>[4x]MPFVNKQFNYKDPVNGVDIAYIKIPNVGVMQPVKAFKIHNKIWVIPERDTFTNPEEGDLNPPPEAKQVPVSYYDSTYLSTDNEKDNY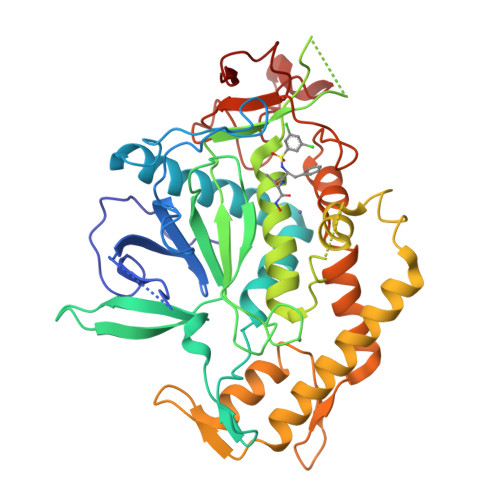LKGVTKLFERIYSTDLGRMLLTSIVRGIPFWGGSTIDTELKVIDTNCINVIQPDGSYRSEELNLVIIGPSADIIQFECKSFGHEVLNLTRNGYGSTQYIRFSPDFTFGFEESLEVDTNPLLGAGKFATDPAVTLAHELIHAGHRLYGIAINPNRVFKVNTNAYYEMSGLEVSFEELRTFGGHDAKFIDSLQENEFRLYYYNKFKDIASTLNKAKSIVGTTASLQYMKNVFKEKYLLSEDTSGKFSVDKLKFDKLYKMLTEIYTEDNFVKFFKVLNRKTYLNFDKAVFKINIVPKVNYTIYDGFNLRNTNLAANFNGQNTEINNMNFTKLK In contrast to E. coli, C. jejuni has only one major outer membrane protein (MOMP), which is thus far present in all isolates and is highly (but not absolutely) conserved in other Campylobacteria. MOMP is an 18-stranded antiparallel β-barrel porin with an elliptical shape common to other 18-stranded porins. Unusually for an 18-stranded β-barrel, MOMP adopts the same trimeric arrangement as seen for OmpF and OmpC, which are 16-stranded β-barrels. The most striking difference between MOMP and OmpF/OmpC from E. coli is the presence of a Ca2 +-binding site in the constriction zone of MOMP.

To allay concerns about the “nativeness” of this recombinant structure arising from the difference in the lipid environment during expression, we also determined the structure of MOMP purified directly from Campylobacter and we found it to be essentially identical. In a different approach, native MOMP was purified from Campylobacter and yielded 1 mg protein per 3 g of C. jejuni cell paste. The protein purified from Campylobacter (nMOMP) was solved via molecular replacement using the recombinant MOMP structure as a search model. Beyond small differences due to crystal packing and resolution, we have not detected any meaningful structural difference between the two proteins (RMSD of 0.45 Å for 398 Cα position using SSM). In the protein purified from Campylobacter, the helix is also present and adopts the same organization but lacks the short strand seen in the overexpressed recombinant protein. The protein purified from Campylobacter was crystallized in the presence of Ca2 + ions and has an ion in an identical position but also has a second ion located outside the barrel at the interface between subunits. The recombinant structure shows a different side-chain conformation, implying that in the recombinant protein, this site does not exist. The identical trimeric arrangement is found in the protein purified from Campylobacter; in this case, the trimer is found in the crystallographic asymmetric unit. We detected no difference in structure or function between the MOMP purified from C. jejuni and the MOMP heterologously expressed in E. coli.

>TPLEEAIKDVDVSGVLRYRYDTGNFDKNFLNNSNLNNSKQDHKYRAQVNFSAAIADNFKAFVQFDYNAVDGGTGVDNATNAEKGLFVRQLYLTYTNEDVATSVIAGKQQLNIIWTDNGVDGLVGTGVKVVNNSIDGLTLAAFAVDSFMAAEQGSDLLGQSTYVGNGKNNNDSFKLDSIGNLYGAAAVGSYDLAGGQFNPQLWLAYWDQVAFFYAVDAAYSTTIFDGINWTLEGAYLGNSLDSELDDKKTYANGNLFALKGSIEVNGWDASLGGLYYGDKEKASTVVIEDQGNLGSLLAGEEIFYTTGSRLNGDTGRNIFGYVTGGYTFNETVRVGADFVYGGTKTEATTHLGGGKKLEAVARVDYKYSPKLNFSAFYSYVNLDQGVNTNESADHSTVRLQALYKF[3x]>[2x]GSHMIKVLSPAKINLGLWVLGRLPSGYHEILTLYQEIPFYDEIYIREGVLRVETNIGIPQEENLVYKGLREFERITGIEINYSIFIQKNIPPGAGLGGGSSNLAVVLKKVNELLGSPLSEEELRELVGSISADAPFFLLGKSAIGRGKGEVLEPVETEISGKITLVIPQVSSSTGRVYSSLREEHFVTPEYAEEKIQRIISGEVEEIENVLGDIARELYPEINEVYRFVEYLGFKPFVSGSGSTVYFFGGASEELKKAAKMRGWKVVELEL

4-Diphosphocytidyl-2C-methyl-d-erythritol kinase (IspE) catalyses the ATP-dependent conversion of 4-diphosphocytidyl-2C-methyl-d-erythritol (CDPME) to 4-diphosphocytidyl-2C-methyl-d-erythritol 2-phosphate with the release of ADP. This reaction occurs in the non-mevalonate pathway of isoprenoid precursor biosynthesis and because it is essential in important microbial pathogens and absent from mammals it represents a potential target for anti-infective drugs. The enzyme displays the characteristic α/β galacto-homoserine-mevalonate-phosphomevalonate kinase fold, with the catalytic centre positioned in a deep cleft between the ATP- and CDPME-binding domains. Gel filtration and analytical ultracentrifugation indicate that AaIspE is a monomer in solution.

Although data for complex I were measured from AaIspE co-crystallized with the relatively stable ATP analogue AMP-PNP only ADP could be modeled. The lack of electron density for the terminal phosphate groups of CDPME2P and AMP-PNP is either a result of disorder and/or hydrolysis. In complex I, CDP displays a single conformation in molecule A and three in molecule B (not shown). Such conformational freedom, distinct from the ordered substrate, may reflect loss of the methylerythritol component and the numerous stabilizing interactions that it forms deep within the enzyme active site. The cytosine moieties of the four CDP molecules interact with Tyr24, His25, Lys145 and Tyr175 with differences (not shown) confined to the orientation and binding modes of the solvent-exposed ribose and phosphate groups. One CDP conformer in molecule B is similar to that observed in molecule A. In the second conformer in molecule B the α-phosphate occupies a similar position but the β-phosphate group is directed out of the active site to interact with both Tyr24 OH and the carbonyl of Ile127. This latter interaction suggests that protonation of the phosphate has occurred. In the third conformer the α-phosphate interacts with the backbone amide of Gly172, the β-phosphate group with the Ser169 carbonyl, Thr171 amide and OG1.> GETGQVIKSAVRSTVENTVQSTHSITTEATPALQAAETGATSNASDESMIETRNVVNTHGVAETSLEAFYGRAGLVAMFSTDGGIYRWYINFGEYVQLRAKLELLTYARFDMEFTIVAQVVNAQSKVQDFNVDYQ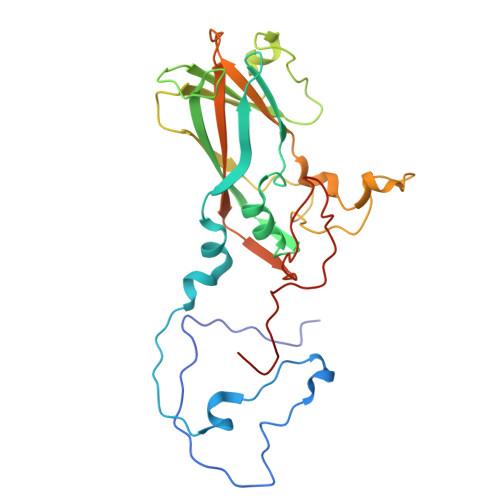VMFVPPGASVPENQDSYQWQSSCNPSVISNTGLPPARVSVPFMSSANAYSFSYDGYTQFGDTSGSSYGIVPSNYLGMLVVRTCEDLDGTRLRVRVYAKPKHVKGWIPRSPRMTPYKSRYTGVYTDTTKFCANRARITTAG>LTFESTSRFAEVDVDGPLKLHYHEAGVGNDQTVVLLHGGGPGAASWTNFSRNIAVLARHFHVLAVDQPGYGHSDKRAEHGQFNRYAAMALKGLFDQLGLGRVPLVGNSL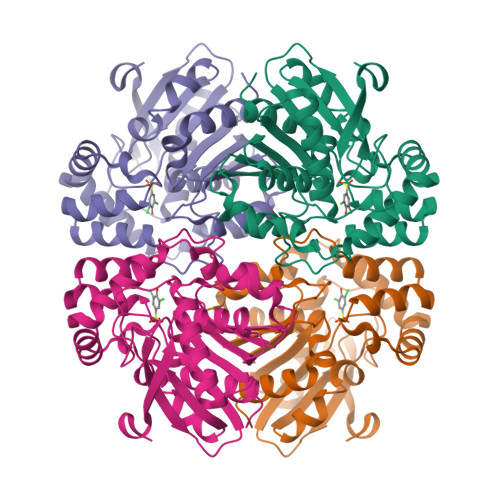GGGTAVRFALDYPARAGRLVLMGPGGLSINLFAPDPTEGVKRLSKFSVAPTRENLEAFLRVMVYDKNLITPELVDQRFALASTPESLTATRAMGKSFAGADFEAGMMWREVYRLRQPVLLIWGREDRVNPLDGALVALKTIPRAQLHVFGQCGHWVQVEKFDEFNKLTIEFLGGG[2x]> MLSNELRQTLQKGLHDVNSDWTVPAAIINDPEVHDVERERIFGHAWVFLAHESEIPERGDYVVRYISEDQFIVCRDEGGEIRGHLNACRHRGMQVCRAEMGNTSHFRCPYHGWTYSNTGSLVGVPAGKDAYGNQLKKSDWNLRPMPNLASYKGLIFGSLDPHADSLEDYLGDLKFYLDIVLDRSDAGLQVVGAPQRWVIDANWKLGADNFVGDAYHTMMTHRSMVELGLAPPDPQFALYGEHIHTGHGHGLGIIGPPPGMPLPEFMGLPENIVEELERRLTPEQVEIFRPTAFIHGTVFPNLSIGNFLMGKDHLSAPTAFLTLRLWHPLGPDKMEVMSFFLVEKDAPDWFKDESYKSYLRTFGISGGFEQDDAENWRSITRVMGGQFAKTGELNYQMGRGVLEPDPNWTGPGEAYPLDYAEANQRNFLEYWMQLMLAESPLRDGNSNGSGTADASTPAAA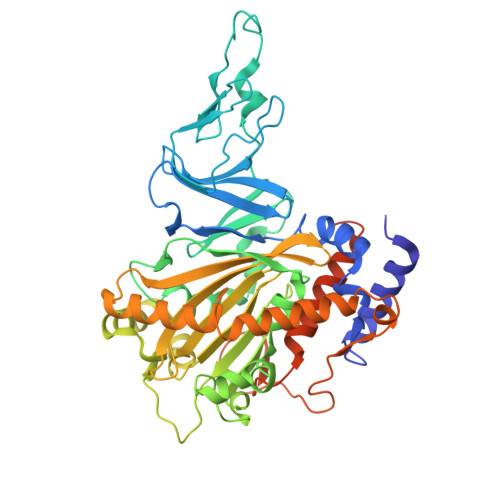KSKSPAKAEA In this study, we identify a family of complement inhibitors from the hard tick Rhipicephalus pulchellus, hereafter termed CirpA (Complement inhibitor from R. pulchellus of the alternative pathway). Functional and structural characterisation reveals that members of the CirpA family directly bind to properdin, inhibiting its ability to promote complement activation, and leading to potent inhibition of the complement response in a species specific manner. Whilst many molecules act to control inappropriate activation, Properdin is the only known positive regulator of the human complement system. All CirpA structures share a lipocalin fold with a short N-terminal α-helix followed by an eight-stranded beta-barrel and a longer C-terminal α-helix.

Using this strategy, we were able to purify CirpA1, A3, A4, and A5 and determine their structure using X-ray crystallography to a resolution of 2.0, 2.1, 1.8, and 1.9 Å respectively. Overall, the structures appear very similar, with the biggest conformational differences in the tilt angle of the C-terminal helix H2 as well as variations in loops between beta strands 4 and 5 (L4-5) and between strands 7 and 8 (L7-8). We identified three regions with high conformational variability between homologs. All these regions are part of the observed binding interface between CirpA1 and properdin, and hence the conformational differences might render other homologs incompatible with binding human properdin. Another CirpA1 residue undergoing a conformational rearrangement upon properdin binding is Y122 which forms a hydrophobic pocket around properdin P377 together with CirpA1 residues F122, Y131, and F150. This pocket is incomplete in all three CirpA1 homolog structures. However, it is likely that the homologues have evolved to target properdin from other species, especially given the identification of multiple CirpA homologues in a single tick species.

>MGNDWNPESFAIDEFMNTTDDIWVLNTTQQNPQACKKDKKHNITENGIYFFRSHKENGQIKTQTLFGEFIHFSEEEKVNNRISISDESSGVHAEHLYYSSEDKKCGLVQVFAKDQNVWTELRVRGHPNYGSLDAGCRREYEAYVKEIKGKKNSTSPYSDDCQIKV[8x]>PA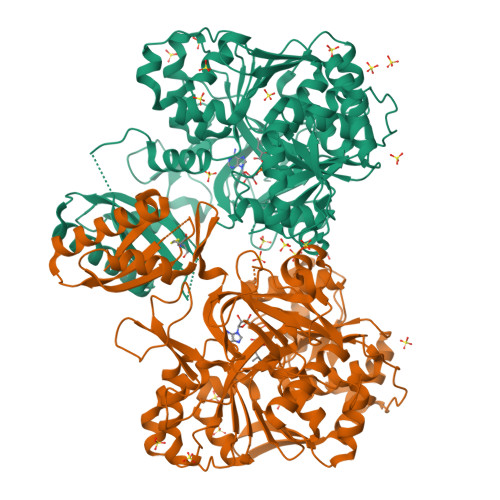LSYGGDLDVTQGAQTLQDVLTEAAKTTNGLTYIVNSKNELTQSYAQLQGDAERVLTGLRALGLKAGDPVFFQFSSNHAMVTAFWACVLGGFVPTLVSAAPTYREMNAAVKKLHHAWKLLEHPLILTDDSLIEEVQGLAFLWHTDQLRVAAVEPMLTLERDTAAHPAAPDDSVFFILTSGSTGMPKCVEHSHRSVLANVKGTVAANQFTQEDVSLDWMPLDHIGGIVMFHLVNVYTGCEQIRARTDDFIAQPLRWLDWMDRYRATKTWAPNFAFAMINDYEKEISSGSWDLSAMTCMINGAEAVVPKTIHRFLHLLAPHGLKGDVIRPAFGMSEISSAVVFSFAIERGDENSGVLTFEETSLTEQLRPAEARETGTVSFTELGKPIPGITIRIVNHQHELLPEDHIGRVQIKGPTTMKGYYRNDEANQEVFQADGWFHTGDLGFLHEGRLTLTGREKDMIIINGKNYHNYEIEAIAEEVPGVETSFVAACSVRMEASASDELILFFTPKLYEPAYIMRASQHIKSHIATKMGLSASRIIPVQKHAFPKTSSGKIERAQLKTRWQEGAAAENLYFQ[2x]> SMENILNDINKRFISLPEEDVRGNK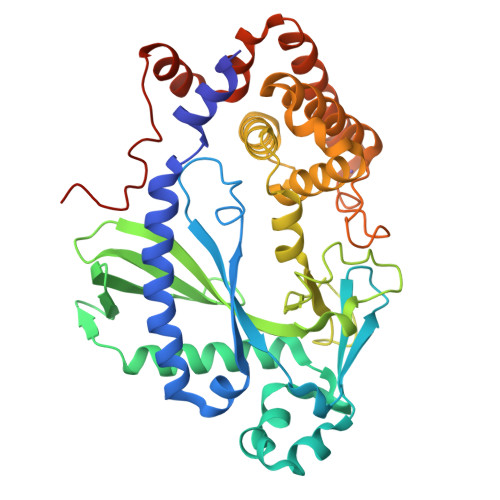QILESVLRTFVEQMKTQDPLFKALFRRVFYGGSFYDGLKVGKPEEFDLDILLHIPIYAQPVLNESNVPGFVWLKLNNLDGWLRQPEGRVYKDFRKKFLADNDFLDTGKTLRWMESLVQKTLNTLPWVNNATCELTNEFGTFHINWWKGGPAMTLGISHSSGEKIMDVDLVACFVFSGDKWPINGYRSNPFPSTKPEFFIVPKKPQGPVNPQGRYWSLSFQEQERVLIDNKNRLKPAVKLIKKLKEKTHPNIASYYIKTVFLHIIEQKDQSFWNKSLREVFMTTLREYNEFIADQSIPYYWCRKNNLIGHLAPITLNNISNRIGYIIKDIENNPENIAKHLLTKEEYTKYIQGEDVMAEALPALPASQTSSCVII>[2x]MALEEIRPKEVYLDRKLLTLEDKELGSGNFGTVKKGYYQMKKVVKTVAVKILKNEANDPALKDELLAEANVMQQLDNPYIVRMIGICEAESWMLVMEMAELGPLNKYLQQNRHVKDKNIIELVHQVSMGMKYLEESNFVHRD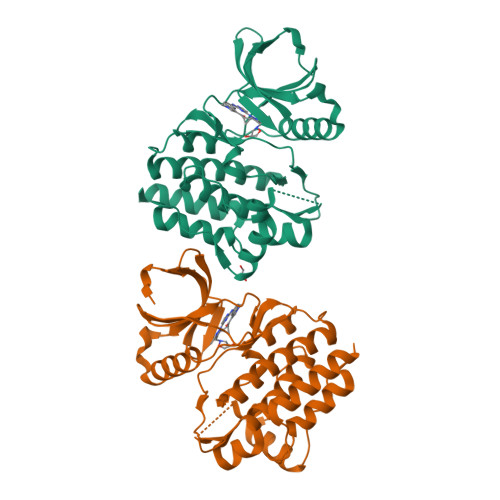LAARNVLLVTQHYAKISDFGLSKALRADENYYKAQTHGKWPVKWYAPECINYYKFSSKSDVWSFGVLMWEAFSYGQKPYRGMKGSEVTAMLEKGERMGCPAGCPREMYDLMNLCWTYDVENRPGFAAVELRLRNYYYDVVNLEHHHHHHHH>[4x]MFDPAEKYKM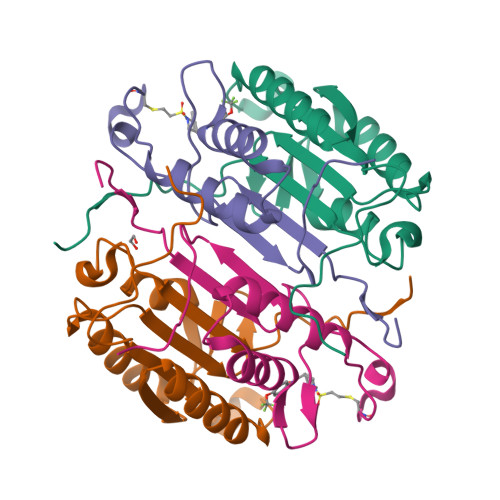DHRRRGIALIFNHERFFWHLTLPERRGTCADRDNLTRRFSDLGFEVKCFNDLKAEELLLKIHEVSTVSHADADCFVCVFLSHGEGNHIYAYDAKIEIQTLTGLFKGDKCHSLVGKPKIFIIQACRGNQHDVPVIPLDVVD;>[4x]MAASVYTLPAGADFLMCYSVAEGYYSHRETVNGSWYIQDLCEMLGKYGSSLEFTELLTLVNRKVSQRRVDFCKDPSAIGKKQVPCFASMLTKKLHFFPKSNLEHHHHHH> MEMAISKAGRRLKAAKKVERKKIVSGPALPGKLADCVGQTREESELFIVEGDSAGGSAKQARDKNFQAIMPIRGKILNTWEVSSDEVLASQEVHDIAIAIGVDPGSDDLSELRYGKICILADADSDGLHIATLLCALFVKHFPALVEEGHLYVAMPPLFRIDIGKDVHYALDDEELETILKNVKGNKNPQITRFKGLGEMNAIQLRETTMDPNTRRLVQLDLDDAHLTAGLLDKLLAKKRAADRKQWLEQKGNLADITVEDKLTMTSLAHHATENRSVAEFTEQAYLNYAMYVIMDRALPHISDGLKPVQRRIVYAMSELGLKSSGKPKKSA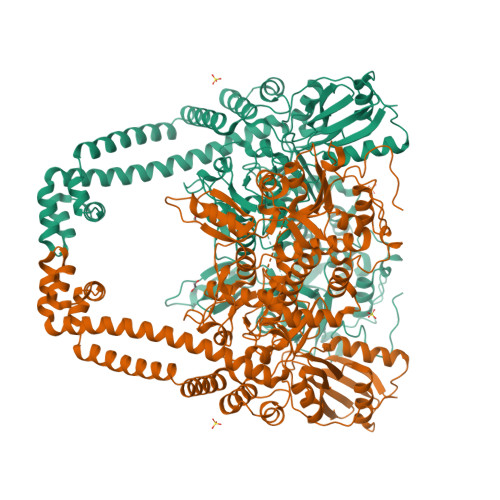RTVGDVLGKYHPHGDSACYEAMVLMAQPFSYRYPLIEGQGNWGSPDDPKSFAAMRYTEAKLSAYSELLLSELGQGTSEWQDNFDGSLKEPITLPARVPNILLNGTTGIAVGMATDIPPHNLREVVKGTIALIRNPQTSDEKLAEYIPAPDLPTKAEIITPPEELLKIQTTGRGSYRMRAVYTIEKNEIVITELPYQVSGSKVITQIADQMQAKKLPLVVDVRDESDHENPTRLVIVLRSNRIDAEAVMSHLFATTDLESSYRVNLNMIGEDGRPQVKSIRRILLEWIEIRKKTVTRRLQYHLNRIEKRLHILAGLLIAYLDIDTVIRIIREEDQPKPVLMEHFNIDEIQAEAILELKLRHLAKLEEMEIRHEQDELSAKAAIIREQLENPESLKNLIISELKEDAKKFGDERRSPIVARAEAVQIKEQDLMPAET>[3x]MATSFDNLLYDLDAATGVLTLTVNRPAKLNALNAATIAELDTAAQ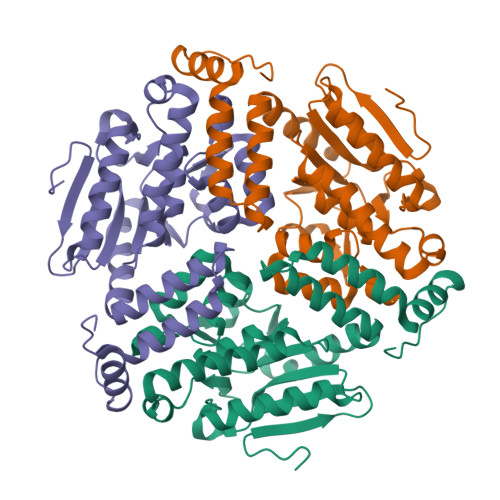QALADPAVRAILLTGSGEKAFVAGADIAELASLTAVQAAGASAYGQRVFAQFERSPKPVVAAVNGFALGGGCELAMACHLRVAADTARFGLPEVSLGLLPGYGGTQRLPQLVGKAKALELMLTADMIKADEALRLGLVNHVVPLAELLGFCQQLLAKMLSKGPVALGLVIECVNAGYDPRQDGYVAETEAFGRAFQTDDFKEGTQAFVEKRPAVFQGK> MHHHHHH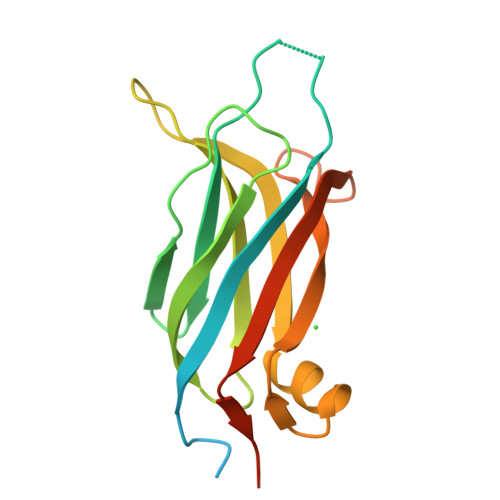SSGRENLYFQGMSDSGSQLGSMGSLTMKSQLQITVISAKLKENKKNWFGPSPYVEVTVDGQSKKTEKCNNTNSPKWKQPLTVIVTPVSKLHFRVWSHQTLKSDVLLGTAALDIYETLKSNNMKLEEVVVTLQLGGDKEPTETIGDLSICLDGLQLESEVVTNGETT>MIAELFTNNALNLVIIFGSCAALILMSFWFRRGNRKRKGFLFHAVQFLIYTIIISAVGSIINYVIENYKLKFITPGVIDFICTSLIAVILTIKLFLLINQFEKQQIKKGRDITSARIMSRIIKITIIVVLVLLYGEHFGMSLSGLLTFGGIGGLAVGMAGKDILSNFFSGIMLYFDRPFSIGDWIRSPDRNIEGTVAEIGWRITKITTFDNRPLYVPNSLFSSISVENPGRMTNRRITTTIGLRYEDAAKVGVIVEAVREMLKNHPAIDQRQTLLVYFNQFADSSLNIMVYCFTKTTVWAEWLAAQQDVYLKIIDIVQSHGADFAFPSQTLYMDNITPPEQGRLEENLYFQ[7x]

To prevent cell lysis, bacteria have mechanosensitive channels that are gated in response to the elevated membrane tension and release solutes, restoring the turgor within the cells. One of the medium-sized paralogues is called YnaI, with 5 TM helices. Structural studies have shown that the main difference between YnaI and MscS are extended sensor paddles, which create a periplasmic indentation in YnaI, and much smaller portals in the vestibule that provide the cytoplasmic access to the pore. The TM paddles are in contact with the surrounding membrane and are therefore responsible for sensing the membrane tension, while the vestibule with the pore formed by the TM3 helices conveys conductivity and selectivity.

Closed YnaI was purified for structure determination by electron cryo-microscopy in n-dodecyl-β-maltoside (DDM) supplemented with 0.5 mg/ml Azolectin (condition I+ ), resulting in a 2.2 Å map. The model built from residues 3–334 resembled the one of YnaI purified in LMNG by Hu et al. with minor differences in the outermost TM helix (TM(−2)), which is frame shifted by 3 residues. In our model, Trp29 in TM(−2) is at the cytosolic interface of the membrane. We found that each sensor paddle has four TM helices that are interconnected by 1-2 hydrogen bonds to the adjacent paddle helix. For example, Asn8 in TM(−2) makes a hydrogen bond with Tyr63 in TM(−1). This hydrogen bonding network suggests that the whole paddle forms a rigid entity within the membrane. In the lipid supplemented YnaI, we could model eight C12 chains, representing alkyl chains, per subunit in the respective densities in the cytosolic pockets, yet we could not distinguish whether they were contributed by detergent or lipid. The eight alkyl chains formed parallel bundles with relative orientations that were compatible with four phospholipid molecules in a membrane context. Thus, the dispersed alkyl chain bundles were part of a hydrophobic inter-subunit interaction network that was located between the transmembrane part and the vestibule outside of the plane of the membrane. In the closed but not open conformation, the pore lining Met158 interacts with Met158 of one adjacent subunit and with Lys161 of the other adjacent subunit.>STTDQPLAKDKVALLIGNMNYREHPKLKAPLVDVYELTNLLRQLDFKVVSLLDLTEYEMRNAVDEFLLLLDKGVYGLLYYAGHGYENFGNSFMVPVDAPNPYRSENCLCVQNILKLMQEKETGLNVFLLDMCRKRNDYDDTIPILDALKVTANIVFGYATCQGAEAFEIQHSGLANGIFMKFLKDRLLEDKKITVLLDEVAEDMGKCHLTKGKQALEIRSSLSEKRALTDPIQGTEYSAESLVRNLQWAKAHELPESMCLKFDCGVQIQLGFAAEFSNVM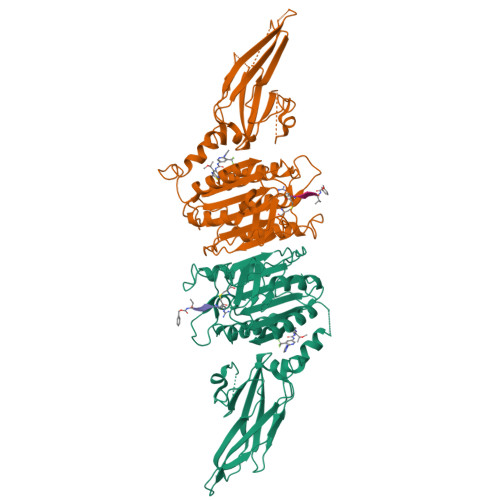IIYTSIVYKPPEIIMCDAYVTDFPLDLDIDPKDANKGTPEETGSYLVSKDLPKHCLYTRLSSLQKLKEHLVFTVCLSYQYSGLEDTVEDKQEVNVGKPLIAKLDMHR[6x]> EDGKPVWAPHPTDGFQVGNIVDIGPDSLTIEPLNQKGKTFLALINQVFPAEEDSKKDVEDNCSLMYLNEATLLHNIKVRYSKDRIYTYVANILIAVNPYFDIPKIYSSETIKSYQGKSLGTMPPHVFAIADKAFRDMKVLKLSQSIIVSGESGAGKTENTKFVLRYLTESYGTGQDIDDRIVEANPLLEAFGNAKTVRNNNSSRFGKFVEIHFNEKSSVVGGFVSHYLLEKSRICVQGKEERNYHIFYRLCAGASEDIRERLHLSSPDNFRYLNRGCTRYFANKETDKQILQNRKSPEYLKAGSLKDPLLDDHGDFIRMCTAMKKIGLDDEEKLDLFRVVAGVLHLGNIDFEEAGSTSGGCNLKNKSTQALEYCAELLGLDQDDLRVSLTTRVMLTTAGGAKGTVIKVPLKVEQANNARDALAKTVYSHLFDHVVNRVNQCFPFETSSYFIGVLDIAGFEYFEHNSFEQFCINYC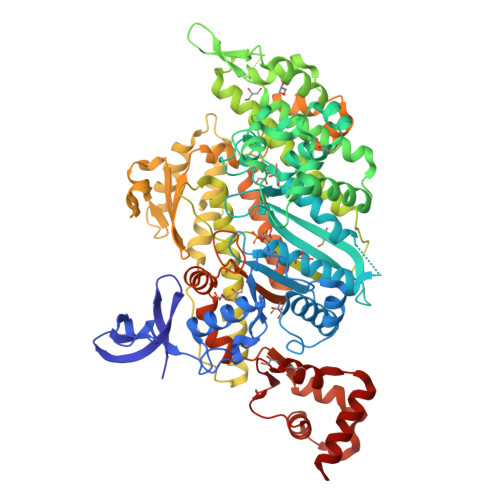NEKLQQFFNERILKEEQELYQKEGLGVNEVHYVDNQDCIDLIEARLVGILDILDEENRLPQPSDQHFTSAVHQKHKDHFRLSIPRKSKLAIHRNIRDDEGFIIRHFAGAVCYETTQFVEKNNDALHMSLESLICESRDKFIRELFESSTNNNKDTKQKAGKLSFISVGNKFKTQLNLLLDKLRSTGASFIRCIKPNLKMTSHHFEGAQILSQLQCSGMVSVLDLMQGGFPSRASFHELYNMYKKYMPDKLARLDPRLFCKALFKALGLNEIDYKFGLTKVFFRPGKFAEFDQIMKSDPDHLAELVKRVNHWLI> QDLALSCGTSEASADQDKKKWEPDTKFLKTGNSIHATATYQDPSLLSTVPYMTARIFTAPATYEIPIKGDKRHLLRLYFYPSTYTGLNISNSYFTVEANDVTLLSNFSAAITCQALTQAYLVKEYSLAPTDKDVLSIKFTPSDKYRDAFAFINGIEVIQMPELFDTAALVGFTDQTMDAKTANLQSMFRLNVGGQDIPGSQDSGGLTRTWYNDAPYIFSAGLGVTLQASNNFRINYQNMPVSIAPADIYKTARSQGPNGDINLKSNLTWMFQIDKNFTYILRLHFCEFQLSKINQKVFNIYINNRTAQADTTPADIIGWTGEKGIPMYKDYAIYVDANNGGEEITLQMTPSTFGQPEYYDSSLNGLEIFKMDTMKNLAGPNPEP;> DLALSCGTSEASADQDKKKWEPDTKFLKTGNSIHATATYQDPSLLSTVPYMTARIFTAPATYEIPIKGDKRHLLRLYFYPSTYTGLNISNSYFTVEANDVTLLSNFSAAITCQALTQAYLVKEYSLAPTDKDVLSIKFTPSDKYRDAFAFINGIEVIQMPELFDTAALVGFTDQTMDAKT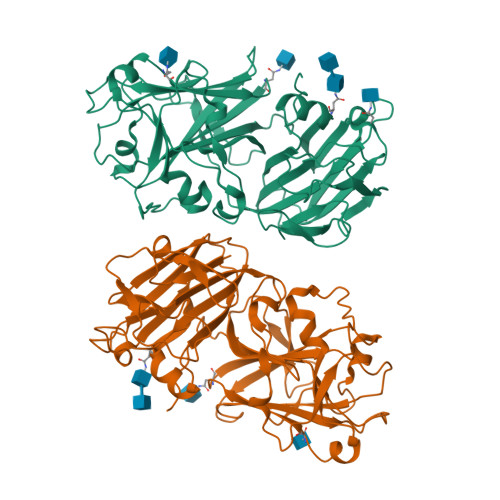ANLQSMFRLNVGGQDIPGSQDSGGLTRTWYNDAPYIFSAGLGVTLQASNNFRINYQNMPVSIAPADIYKTARSQGPNGDINLKSNLTWMFQIDKNFTYILRLHFCEFQLSKINQKVFNIYINNRTAQADTTPADIIGWTGEKGIPMYKDYAIYVDANNGGEEITLQMTPSTFGQPEYYDSSLNGLEIFKMDTMKNLAGPNPEP S. pneumoniae produces up to three distinct sialidase enzymes: NanA, NanB, and NanC. NanC is an unusual sialidase in that its primary reaction product is 2-deoxy-2,3-didehydro-N-acetylneuraminic acid (Neu5Ac2en, also known as DANA), a nonspecific hydrolytic sialidase inhibitor. NanC adopts the same overall topology as seen in NanA and NanB, with a CBM (residues 85–271), followed by a catalytic domain (residues 272–740). The catalytic domain adopts the canonical glycoside hydrolase family 33 sialidase, six-bladed β-propeller fold shared by viral, bacterial, and mammalian sialidases.

The production of Neu5Ac2en from α2–3-linked sialosides by the catalytic domain is confirmed within a crystal structure. However, when NanC crystals were soaked with 3′SL, Neu5Ac2en is found in the active site. When longer soaks were performed, Neu5Ac2en is still observed in the active site, and cleaved Neu5Ac was observed in the CBM binding site. When the pool of substrate is exhausted and Neu5Ac2en is in excess, NanC can hydrate Neu5Ac2en to Neu5Ac. Thus we propose that Asp-315 abstracts the proton directly from the C3 position, eliminating Tyr-695 and forming Neu5Ac2en. First, Asp-315 is ∼1 Å closer to the C2 of Neu5Ac2en than the equivalent residue in NanA and NanB. This advanced position would allow the C3 proton to be abstracted directly.

>[2x]ETPVLEKNNVTLTGGGENVTKELKDKFTSGDFTVVIKYNQSSEKGLQALFGISNSKPGQQNSYVDVFLRDNGELGMEARDTSSNKNNLVSRPASVWGKYKQEAVTNTVAVVADSVKKTYSLYANGTKVVEKKVDNFLNIKDIKGIDYYMLGGVKRAGKTAFGFNGTLENIKFFNSALDEETVKKMTTNAVTGHLIYTANDTTGSNYFRIPVLYTFSNGRVFSSIDARYGGTHDFLNKINIATSYSDDNGKTWTKPKLTLAFDDFAPVPLEWPREVGGRDLQISGGATYIDSVIVEKKNKQVLMFADVMPAGVSFREATRKDSGYKQIDGNYYLKLRKQGDTDYNYTIRENGTVYDDRTNRPTEFSVDKNFGIKQNGNYLTVEQYSVSFENNKKTEYRNGTKVHMNIFYKDALFKVVPTNYIAYISSNDHGESWSAPTLLPPIMGLNRNAPYLGPGRGIIESSTGRILIPSYTGKESAFIYSDDNGASWKVKVVPLPSSWSAEAQFVELSPGVIQAYMRTNNGKIAYLTSKDAGTTWSAPEYLKFVSNPSYGTQLSIINYSQLIDGKKAVILSTPNSTNGRKHGQIWIGLINDDNTIDWRYHHDVDYSNYGYSYSTLTELPNHEIGLMFEKFDSWSRNELHMKNVVPYITFKIEDLKKNL Seven cell shape-determining genes (csd1, csd2, csd3/hdpA, ccmA, csd4, csd5 and csd6) have been identified in H. pylori. Among them, Csd3 (also known as HdpA) is a bifunctional enzyme. Its d,d-endopeptidase activity cleaves the d-Ala4-mDAP3 peptide bond between cross-linked muramyl tetrapeptides and pentapeptides.

Among these, only the N-terminally 41-residue truncated Csd3 (Csd3Δ41) comprised of residues 42–403 was expressed in soluble form, and it yielded two different forms (the orthorhombic form 1 and the hexagonal form 2) of well diffracting crystals. The form 1 crystal contains two monomers (chains A and B) of Csd3Δ41 in the asymmetric unit. Chains A and B are related by non­crystallographic twofold symmetry. Chains A and B are highly similar to each other, with an r.m.s. deviation of 0.67 Å for 359 Cα atoms. However, they show larger structural deviations from the chain of the form 2 crystal, with r.m.s. deviations of 1.61 and 1.85 Å for 353 Cα atoms in chains A and B, respectively. In the form 1 crystal, the two monomers in the asymmetric unit bury a relatively large surface area of 1130 Å2 per monomer (6.0% of the monomer surface area), whereas the largest buried surface area in the form 2 crystal is 710 Å2 per monomer (3.8% of the monomer surface area). Loop I of Csd3 shows the most significant deviation among the homologues. In form 1 crystals, it is involved in crystal-packing interactions by forming sulfate-mediated salt bridges. Interestingly, the side chain of His339 of Csd3, the first histidine of the HxH motif, shows two different orientations. However, it is flipped about 104° towards the solvent in the form 1 crystals.

>MERLVWDKLTLLGFLEKNHIPQKLYYNLSSQDKELSAEIQSNVTYYTLRDANNTLIQALIPISQDLQIHIYKKGEDYFLDFIPIIFTRKEKTLLLSLQTSPYQDIIKATNDPLLANQLMNAYKKSVPFKRLVKNDKIAIVYTRDYRVGQAFGQPTIKMAMVSSRSNQYYLFSHSNGHYYDSKAQEVAGFLLETPVKYTRISSPFSYGRFHPVLKVRRPHYGVDYAAKHGSLIHSASDGRVGFMGVKAGYGKVVEIHLNELRLVYAHMSAFANGLKKGSFVKKGQIIGRVGSTGLSTGPHLHFGVYKNSRPINPLGYIRTAKSKLHGKQREVFLEKAQRSKQKLEELLKTHSFEKNSFYLLEGFLEHHHHHH[2x]> GNDEYKKDSPSAANPVEPIGASLEDFSIEQLPAKTIYALGENIDLTGLNVTGKYDDGKQRPVKVTSEQISGFSSSVPVDKQEVTITIEGKQ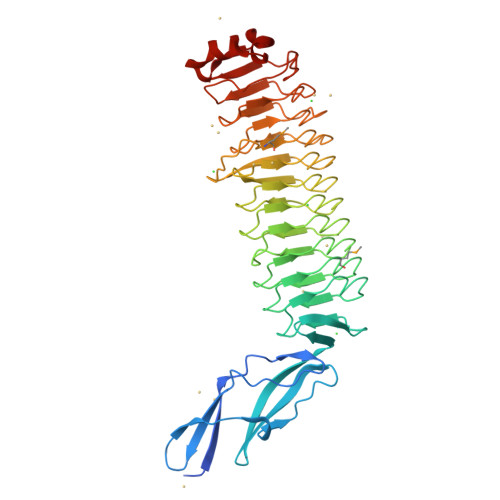KSFSVHISPVRVENGVLTEILKGYNEIILPNSVKSIPKDAFRNSQIAKVVLNEGLKSIGDMAFFNSTVQEIVFPSTLEQLKEDIFYYCYNLKKADLSKTKITKLPASTFVYAGIEEVLLPVTLKEIGSQAFLKTSQLKTIEIPENVSTIGQEAFRESGITTVKLPNGVTNIASRAFYYCPELAEVTTYGSTFNDDPEAMIHPYCLEGCPKLARFEIPESIRILGQGLLGGNRKVTQLTIPANVTQINFSAFNNTGIKEVKVEGTTPPQVFEKVWYGFPDDITVIRVPAESVEKYKNANGWRDFTNKITTF> EQCGRQAGGK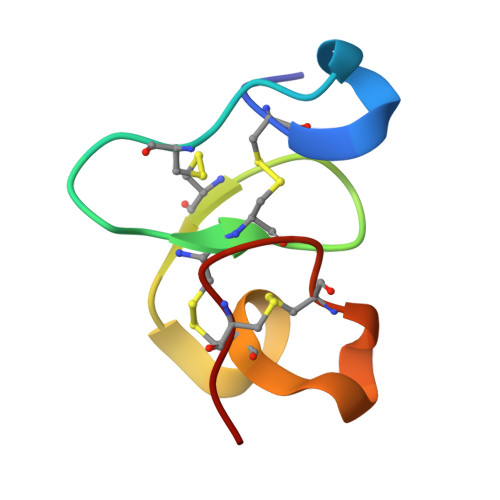LCPDNLCCSQWGWCGSTDEYCSPDHNCQSNCKD>MSAFDGVENQMNGPDSSPRLSQDPREPRSLLSSSCFPITLKFVDVCYRVKIHGMSNDSCNIKKLLGLKQKPSDETRSTEERTILSGVTGMISPGEFMAVLGPSGSGKSTLLNAVAGRLHGSNLTGKILINDGKITKQTLKRTGFVAQDDLLYPHLTVRETLVFVALLRLPRSLTRDVKLRAAESVISELGLTKCENTVVGNTFIRGISGGERKRVSIAHELLINPSLLVLDEPTSGLDATAALRLVQTLAGLAHGKGKTVVTSIHQPSSRVFQMFDTVLLLSEGKCLFVGKGRDAMAYFESVGFSPAFPMNPADFLLDLANGVCQTDGVTEREKPNVRQTLVTAYDTLLAPQVKTCIEVSHFPQDNARFVKTRVNGGGITTCIATWFSQLCILLHRLLKERRHESFDLLRIFQVVAASILCGLMWWHSDYRDVHDRLGLLFFISIFWGVLPSFNAVFTFPQERAIFTRERASGMYTLSSYFMAHVLGSLSMELVLPASFLTFTYWMVYLRPGIVPFLLTLSVLLLYVLASQGLGLALGAAIMDAKKASTIVTVTMLAFVLT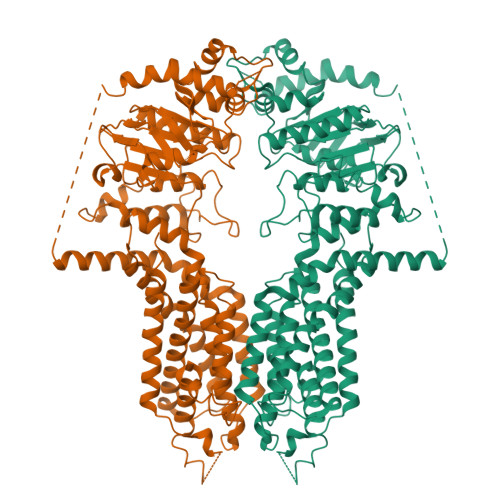GGYYVNKVPSGMVWMKYVSTTFYCYRLLVAIQYGSGEEILRMLGCDSKGKQGASAATSAGCRFVEEEVIGDVGMWTSVGVLFLMFFGYRVLAYLALRRIKH[2x]>[2x]MIVRSFIYEPFQIPSGSMMPTLLIGDFILVEKF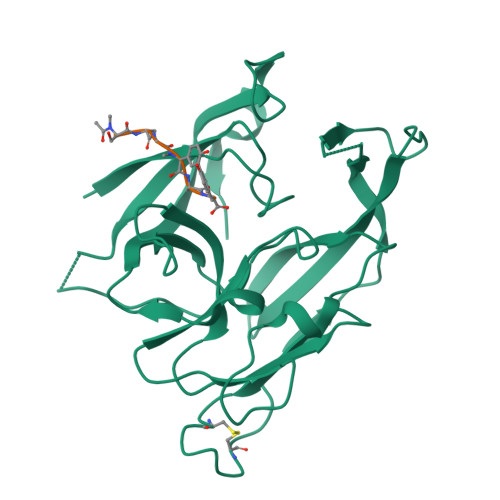AYGIKDPIYQKTLIETGHPKRGDIVVFKYPEDPKLDYIKRAVGLPGDKVTYDPVSKELTIQPGCSSGQACENALPVTYSNVEPSDFVQTFSRRNGGEATSGFFEVPKNETKENGIRLSERKETLGDVTHRILTVPIAQDQVGMYYQQPGQQLATWIVPPGQYFMMGDNRDNSADSRYWGFVPEANLVGRATAIWMSFDKQEGEWPTGLRLSRIGGIH;>[2x]SAGGAY>[4x]GMTQHITRMRREIDEIPEAVQRLLDHGAQDVARVAAVLRLRDPSFVATVARGSSDHVCTYLSYAAELLLGLPVASLGPSVASVYDARLRLDRALCLAVSQSGKSPDIVAMTRNAGRDGALCVALTNDAASPLAGVSAHTIDIHAGPELSVAATKTFVTSAVAGLMLLADWAEDDGLRAALGNLPETLAAASRIDWP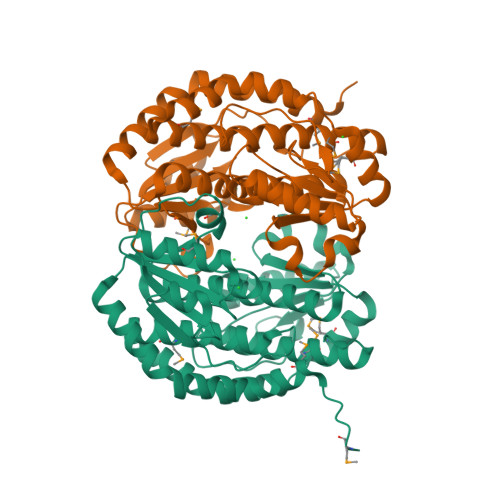EMRVAIGARPSLFTLGRGTSLAVSNEAALKFKETCQLHAESYSSAEVLHGPVSIVEEGFPVLGFAAGDAAEAPLAEIADQIAAKGATVFATTGRVTRARVLEHVRSGHALTDPLSLIVSFYSMVEAFASERGIDPDAPRHLNKVTETV>[4x]SNAEKSRSSWIKQLNASLDEIDPEVADIIELEKARQWKGFELIPSENFTSLSVMQAVGSVMTNKYSEGYPGARYYGGNEYIDMAETLCQKRALEAFQLDPSKWGVNVQSLSGSPANFQVYTALLKPHERIMALDLPHGGHLSHGYQTDTKKISAVSIFFETMPYRLDENTGYIDYDQLEKSAVLFRPKLIVAGASAYARLYDYARIRKVCNKQKAVMLADMAHISGLVAAGVIPSPFEYADVVTTTTHKSLRGPRGAMIFFRKGLKEINKQGKEVMYDYEDRINQAVFPGLQGGPHNHTITGLAVALKQARTPEYKAYQDQVLRNCSKFAETLLAKGYDLVSGGTDNHLVLVNLKNKGIDGSRVEKVLELVHIAANKNTVPGDVSAMVPGGIRMGTPALTSRGFIEEDFAKVAEYFDLAVKIALKIKAESQGTKLKDFVATMQSNEKLQSEMSKLREMVEEYAKQFPTIGFEKETMRYKE

Serine hydroxymethyltransferase (SHMT) reversibly interconverts serine and tetrahydrofolate (THF) into glycine and 5,10-methylene-THF (5,10-meTHF). Next, we have obtained high resolution crystal structures of AtSHMT2 complexed with MTX and PTX, as well as of AtSHMT4-MTX complex. For clarity, in this work we divide THF, MTX, and PTX molecules into three moieties: (i) pteridine or its mimic (P-moiety); (ii) benzoyl (B-moiety); and (iii) glutamate (E-moiety).

Interfaces between subunits A/B and C/D are much more extensive than e.g. between A and D. In the crystal structure of AtSHMT2-MTX complex, we noted two binding modes of MTX, one corresponding to external PLP-Ser aldimine state (EA-type; chains A, B, C) and the other to PLP internal aldimine + free serine state (IA-type; chain D). In this case, direct hydrogen bonds dock exocyclic N4 of MTX to Oε of Glu104* (an asterisk indicates a residue from another, tightly bound subunit), and N2 of MTX to backbone O of Lys414. A network of water-mediated hydrogen bonds link the antifolate to Thr416, Ala423, and Glu104*. Altogether, five out of six heteroatoms of the P-moiety (pteridine-2,4-diamine) participate in hydrogen bonding. Tyr111* π-stacks with the pteridine ring. B-moiety is sandwiched by the side chains of Ile189 and Tyr182 from one side and Ala423 from the other side. The IA-type binding mode (chain D) is characterized by fewer H-bonds. In the P-moiety, exocyclic N2 H-bonds to carbonyl O of Tyr111* and to Nζ of Lys414. The pteridine ring is again stacked with the side chain of Tyr111*, however, it is rotated by 66° with respect to the ring in the EA-type binding. The two Oε atoms of the E-moiety are also involved in binding; Oε1 to the backbone amide of Asp185 and to (apparently protonated) Oδ of Asp185, whereas Oε2 interacts with Nη of Arg223 from the A-chain.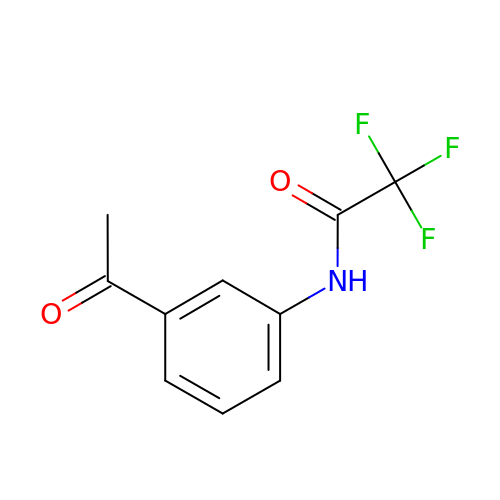~{N}-(3-ethanoylphenyl)-2,2,2-tris(fluoranyl)ethanamide | C10 H8 F3 N O2 | QJIHIZOVLAWHFM-UHFFFAOYSA-N> AAEAAVTQSPRNKVAVTGEKVTLSCQQTNNHNNMYWYRQDTGHGLRLIHYSYGVGNTEKGDIPDGYEASRPSHEQFSLILVSATPSQS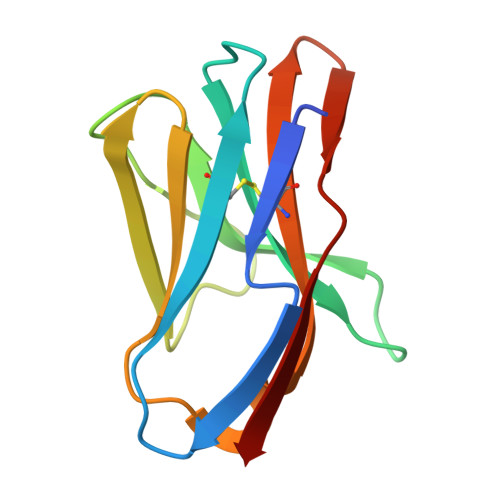SVYFCASGVGGTLYFGAGTRLSVL> ALDTTWKEATLPQVKAMLEKDTGKVSGDTVTYSGKTVHVVAAAVLPGFPFPSFEVHDKKNPTLEIPAGATVDVTFINTNKG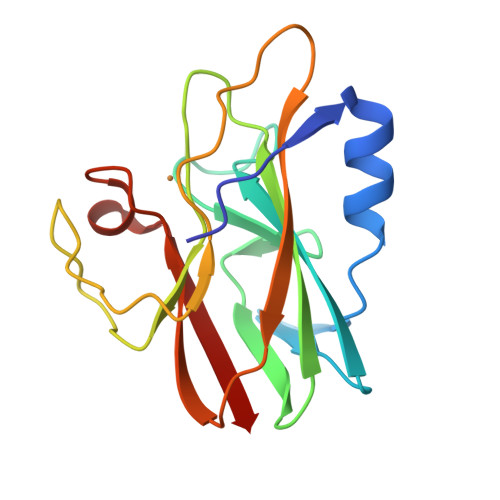FGHSFDITKKGPPYAVMPVIDPIVAGTGFSPVPKDGKFGYTDFTWHPTAGTYYYVCQIPGMAATGMFGKIVVK> MTVPYLNSNRNVASYLQSNSSQEKTLKERFSEIYPIHAQDVRQFVKEHGK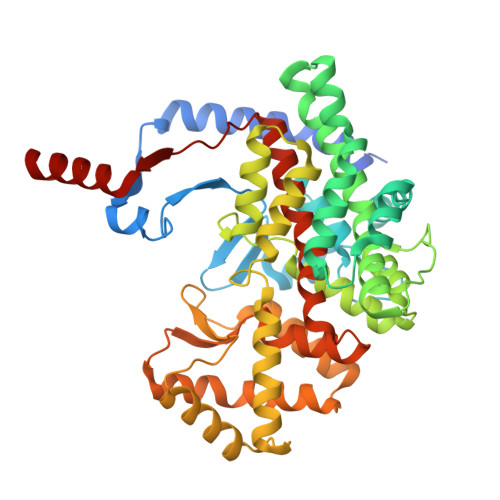TKISDVLLEQVYGGMRGIPGSVWEGSVLDPEDGIRFRGRTIADIQKDLPKAKGSSQPLPEALFWLLLTGEVPTQAQVENLSADLMSRSELPSHVVQLLDNLPKDLHPMAQFSIAVTALESESKFAKAYAQGISKQDYWSYTFEDSLDLLGKLPVIAAKIYRNVFKDGKMGEVDPNADYAKNLVNLIGSKDEDFVDLMRLYLTIHSDHEGGNVSAHTSHLVGSALSSPYLSLASGLNGLAGPLHGRANQEVLEWLFALKEEVNDDYSKDTIEKYLWDTLNSGRVIPGYGHAVLRKTDPRYMAQRKFAMDHFPDYELFKLVSSIYEVAPGVLTEHGKTKNPWPNVDAHSGVLLQYYGLKESSFYTVLFGVSRAFGILAQLITDRAIGASIERPKSYSTEKYKELVKNIESKL> GLPVCGETCVG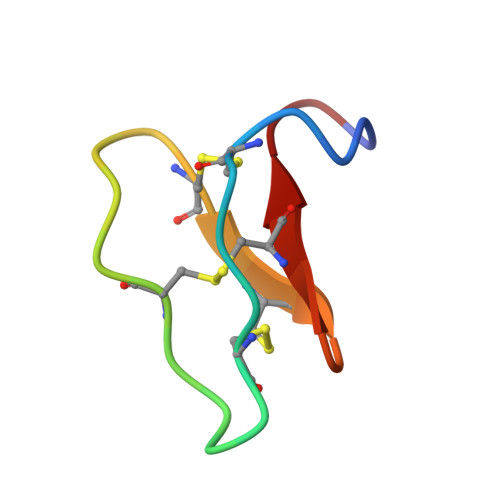GTCNTPGCTCSWPVCTRN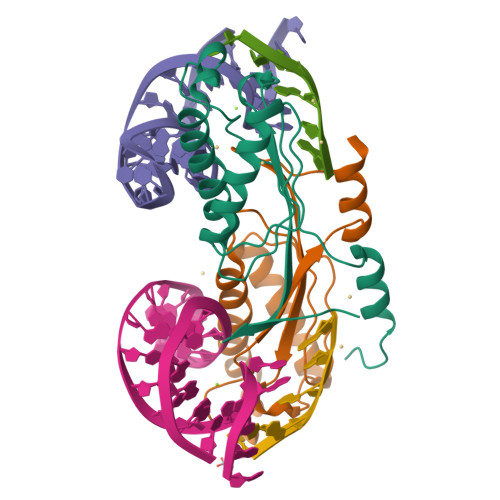>MTYVILPLEMKKGRGYVYQLEYHLIWCVKYRHQVLVGEVADGLKDILRDIAAQNGLEVITMEVMPDHVHLLLSATPQQAIPDFVKALKGASARRMFVAYPQLKEKLWGGNLWNPSYCILTVSENTRAQIQKFIESQHDKE[2x]>[4x]TEST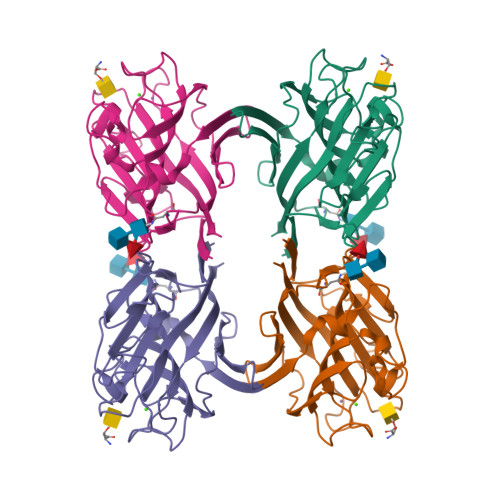SFSFTNFNPNQNNLILQEDALVNSAGTLELTAVAAGAPVPDSLGRALYAAPIHIHDNTTLASFTTSFSFVMAAPAAAAVADGLAFFLAPPDTQPQARGGFLGLFADRAHDASYQTVAVEFDTYSNAWDPNYTHIGIDTNGIESKKTTPFDMVYGEKANIVITYQASTKALAASLVFPVSQTSYAVSARVDLRDILPEYVRVGFSATTGLNAGVVETHDIVSWSFAVSLA3-[[2,4-bis(trifluoromethyl)phenyl]methyl]-5-(hydroxymethyl)-1~{H}-imidazole-2-thione | C13 H10 F6 N2 O S | 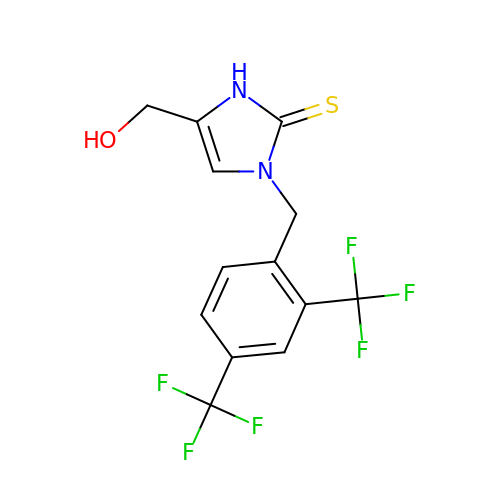WXKONROFPLKHOA-UHFFFAOYSA-N>GSQIPASEQETLVRPKPLLLKLLKSVGAQKDTYTMKEVLFYLGQYIMTKRLYDEKQQHIVYCSNDLLGDLFGVPSFSVKEHRKIYTMIY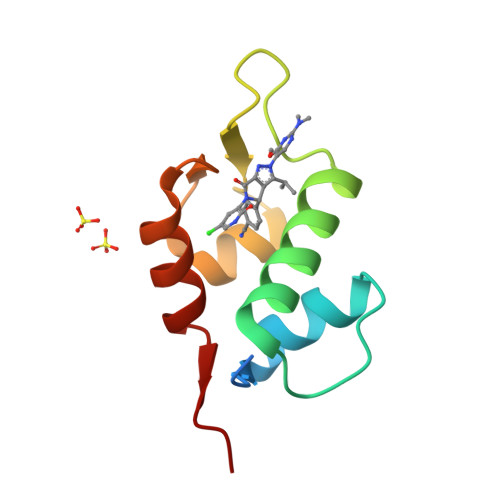RNLVVVN[2x]uridine-5'-diphosphate-3-O-(R-3-hydroxymyristoyl)-N-acetyl-D-glucosamine | C31 H53 N3 O19 P2 | 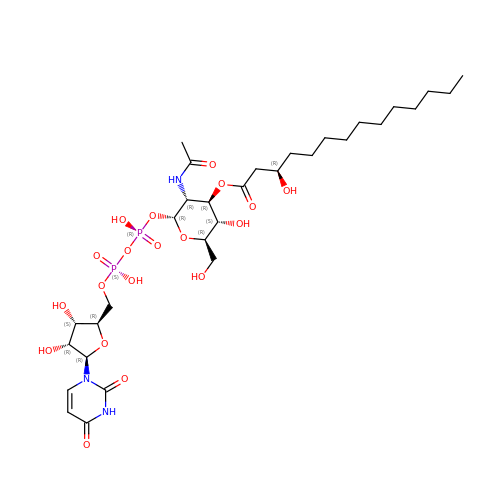TZSJGZGYQDNRRX-MPLCHSTDSA-N>[4x]MSASIPDIKLSSGHLMPSIGFGCWKLANATAGEQVYQAIKAGYRLFDGAEDYGNEKEVGDGVKRAIDEGLVKREEIFLTSKLWNNYHDPKNVETALNKT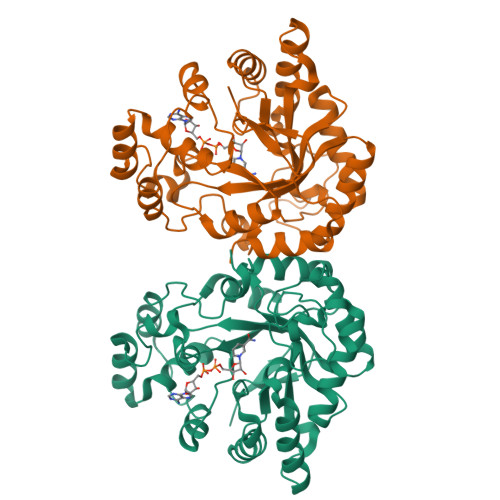LADLKVDYVDLFLIHFPIAFKFVPIEEKYPPGFYCGDGNNFVYEDVPILETWKALEKLVAAGKIKSIGVSNFPGALLLDLLRGATIKPAVLQVEHHPYLQQPKLIEFAQKAGVTITAYSSFGPQSFVEMNQGRALNTPTLFAHDTIKAIAAKYNKTPAEVLLRWAAQRGIAVIPRSDLPERLVQNRSFNTFDLTKEDFEEIAKLDIGLRFNDPWDWDNIPIFV>MSRFQSLLCFVLVSLAAVANAAIGPVADLTLTNAAVSPDGFSREAVVVNGVTPAPLISGQKGDRFQLNVIDNLTNHTMLKTTSIHWHGFFQHGTNWADGPAFVNQCPIASGHSFLYDFQVPDQAGTFWYHSHLSTQYCDGLRGPFVVYDPNDPQASLYDID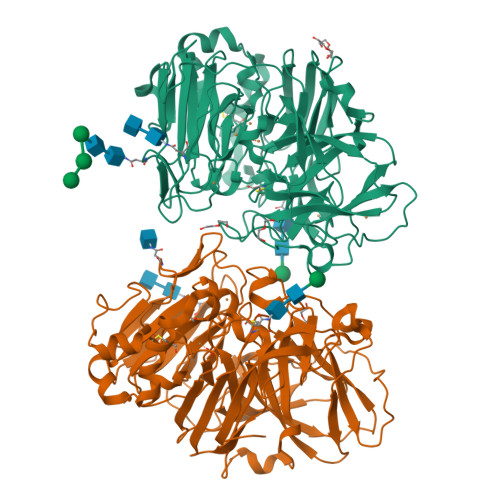NDDTVITLADWYHVAAKLGPRFPPGSDATLINGLGRSPGTTAADLAVIKVTQGKRYRFRLVSLSCDPNHTFSIDGHTMTIIEADSVNTQPLEVDSIQIFAAQRYSFVLDASQPVDNYWIRANPSFGNTGFAGGINSAILRYLGAPEIEPTTTQTTPTKPLTEVDLHPLTPMAVPGRPEPGGVDKPLNMVFNFNGTNFFINNHSFVPPSVPVLLQILSGAQAAQDLVPEGSVYVLPSNSSIEISFPATVNAPGAPHPFHLHGHTFAVVRSAGSSEYNYDNPIFRDVVSTGTPGDNVTIRFQTANPGPWFLHCHIDFHLDAGFAVVMAEDTPDTTAANPVPQAWSDLCPIYDALDPSDL[2x]3-[4-(2-HYDROXYETHYL)PIPERAZIN-1-YL]PROPANE-1-SULFONIC ACID | C9 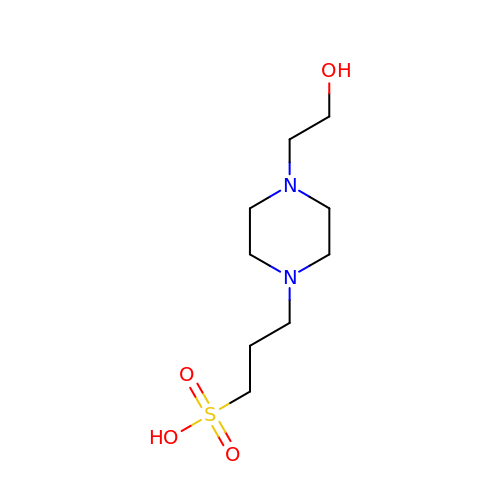H20 N2 O4 S | OWXMKDGYPWMGEB-UHFFFAOYSA-N4-(2-hydroxyethyl)benzene-1,2-diol | C8 H10 O3 | 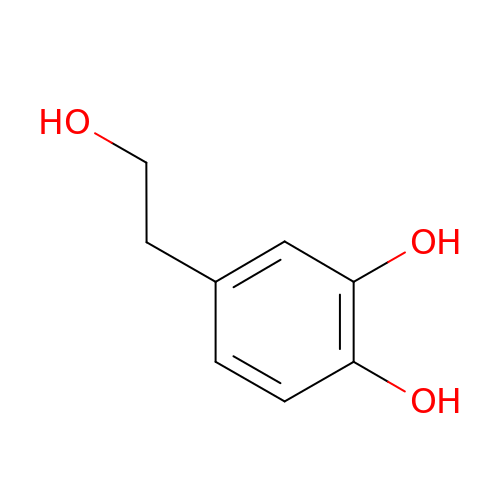JUUBCHWRXWPFFH-UHFFFAOYSA-N>MMVISEKVRKALNDQLNREIYSSYLYLSMATYFDAEGFKGFAHWMKKQAQEELTHAMKFYEYIYERGGRVELEAIEKPPSNWAGIKDAFEAALKHEEFVTQSIYNILELASEEKDHATVSFLKWFVDEQVEEEDQVREILDLLEKAYGQ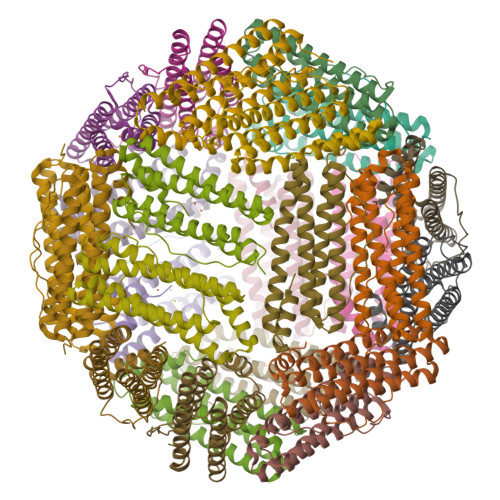MSVIFQLDRYLGQRE[8x]> RVCGVSAARLTPCGTGTSTDVVYRAFDIYNDKVAGFAKFLKTNCCRFQEKDEDDNLIDSYFVVKRHTFSNYQHEETIYNLLKDCPAVAKHDFFKFRIDGDMVPHISRQRLTKYTMADLVYALRHFDEGNCDTLKEILVTYNCCDDDYFNKKDWYDFVENPDILRVYANLGERVRQALLKTVQFCDAMRNAGIVGVLTLDNQDLNGNWYDFGDFIQTTPGSGVPVVDSYYSLLMPILTLTRALTAESHVDTDLTKPYIKWDLLKYDFTEERLKLFDRYFKYWDQTYHPNCVNCLDDRCILHCANFNVLFSTVFPPTSFGPLVRKIFVDGVPFVVSTGYHFRELGVVHNQDVNLHSSRLSFKELLVYAADPAMHAASGNLLLDKRTTCFSVAALTNNVAFQTVKPGNFNKDFYDFAVSKGFFKEGSSVELKHFFFAQDGNAAISDYDYYRYNLPTMCDIRQLLFVVEVVDKYFDCYDGGCINANQVIVNNLDKSAGFPFNKWGKARLYYDSMSYEDQDALFAYTKRNVIPTITQMNLKYAISAKNRARTVAGVSICSTMTNRQFHQKLLKSIAATRGATVVIGTSKFYGGWHNMLKTVYSDVENPHLMGWDYPKCDRAMPNMLRIMASLVLARKHTTCCSLSHRFYRLANECAQVLSEMVMCGGSLYVKPGGTSSGDATTAYANSVFNICQAVTANVNALLSTDGNKIADKYVRNLQHRLYECL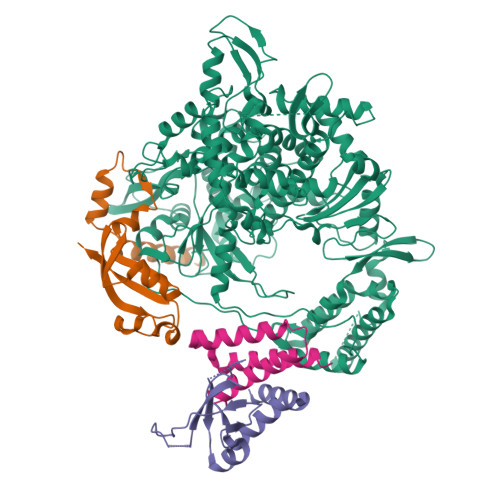YRNRDVDTDFVNEFYAYLRKHFSMMILSDDAVVCFNSTYASQGLVASIKNFKSVLYYQNNVFMSEAKCWTETDLTKGPHEFCSQHTMLVKQGDDYVYLPYPDPSRILGAGCFVDDIVKTDGTLMIERFVSLAIDAYPLTKHPNQEYADVFHLYLQYIRKLHDELTGHMLDMYSVMLTNDNTSRYWEPEFYEAMYTPHTVLQ;>AIASEFSSLPSYAAFATAQEAYEQAVANGDSEVVLKKLKKSLNVAKSEFDRDAAMQRKLEKMADQAMTQMYKQARSEDKRAKVTSAMQTMLFTMLRKLDNDALNNIINNARDGCVPLNIIPLTTAAKLMVVIPDYNTYKNTCDGTTFTYASALWEIQQVVDADSKIVQLSEISMDNSPNLAWPLIVTALRANSAVKLQ[2x];> SKMSDVKCTSVVLLSVLQQLRVESSSKLWAQCVQLHNDILLAKDTTEAFEKMVSLLSVLLSMQGAVDINKLCEEMLDNRATLQ>[4x]MSLDRTTQQPFGNGYLSVEQANLILNHLPLEITFVNKDDIFQYYNDSVPAAEMVFKRTPSQVGRNVELCHPPKVLDKVKKVFELLRNGQRDKVNMWFQSERLGKFVYVTYAAVRDQA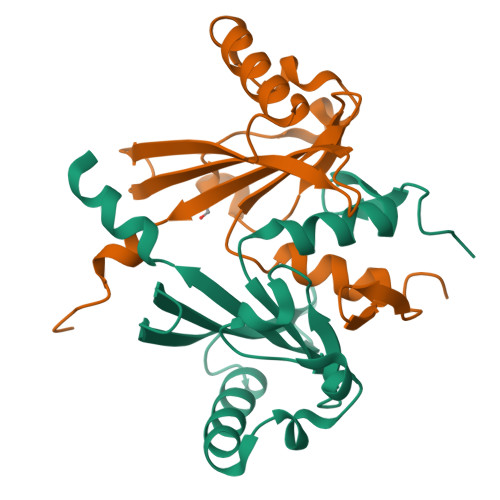GDFQGVLEYVQDIKPFFELDSEFNRDEGHHHHHH> MAMHPRKDWYELTRATNWTPSYVTEEQLFPERMSGHMGIPLEKWESYDEPYKTSYPEYVSIQREKDAGAYSVKAALERAKIYENSDPGWISTLKSHYGAIAVGEYAAVTGEGRMARFSKAPGNRNMATFGMMDELRHGQLQLFFPHEYCKKDRQFDWAWRAYHSNEWAAIAAKHFFDDIITGRDAISVAIMLTFSFETGFTNMQFLGLAADAAEAGDYTFANLISSIQTDESRHAQQGGPALQLLIENGKREEAQKKVDMAIWRAWRLFAVLTGPVMDYYTPLEDRSQSFKEFMYEWIIGQFERSLIDLGLDKPWYWDLFLKDIDELHHSYHMGVWYWRTTAWWNPAAGVTPEERDWLEEKYPGWNKRWGRCWDVITENVLNDRMDLVSPETLPSVCNMSQIPLVGVPGDDWNIEVFSLEHNGRLYHFGSEVDRWVFQQDPVQYQNHMNIVDRFLAGQIQPMTLEGALKYMGFQS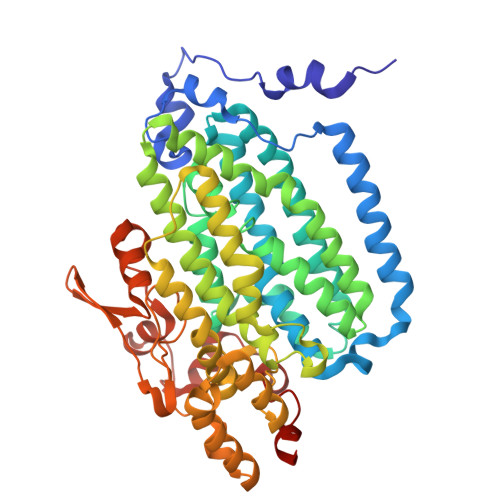IEEMGKDAHDFAWADKCK>[2x]MLLNALASLGHKGIKTLRTFGRAGLMLFNALVGKPEFRKHAPLLVRQLYNVGVLSMLIIVVSGVFIGMVLGLQGYLVLTTYSAETSLGMLVALSLLRELGPVVAALLFAGRAGSALTAEIGLMRATEQLSSMEMMAVDPLRRVISPRFWAGVISLPLLTVIFVAVGIWGGSLVGVSWKGIDSGFFWSAMQNAVDWRMDLVNCLIKSVVFAITVTWISLFNGYDAIPTSAGISRATTRTVVHSSLAVLGLDFVLTALMFGN;>[2x]MEQSVANLVDMRDVSFTRGNRCIFDNISLTVPRGKI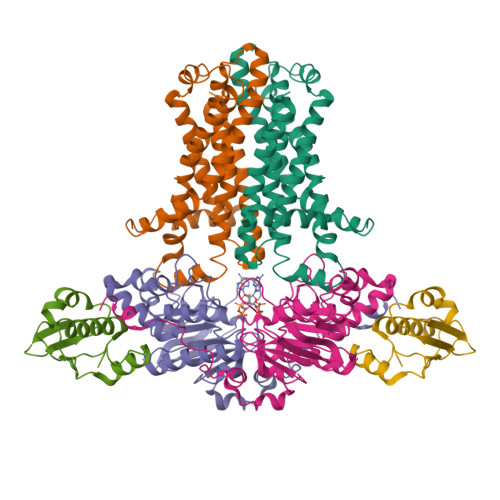TAIMGPSGIGKTTLLRLIGGQIAPDHGEILFDGENIPAMSRSRLYTVRKRMSMLFQSGALFTDMNVFDNVAYPLREHTQLPAPLLHSTVMMKLEAVGLRGAAKLMPSELSGGMARRAALARAIALEPDLIMFDEPFVGQDPITMGVLVKLISELNSALGVTCVVVSHDVPEVLSIADHAWILADKKIVAHGSAQALQANPDPRVRQFLDGIADGPVPFRYPAGDYHADLLPGS;>[2x]MSESLSWMQTGDTLALSGELDQDVLLPLWEMREEAVKGITCIDLSRVSRVDTGGLALLLHLIDLAKKQGNNVTLQGVNDKVYTLAKLYNLPADVLPR>NSALDFLKHHLGAATPENPEIELLRLELAEMKEKYEAIVEENKKLK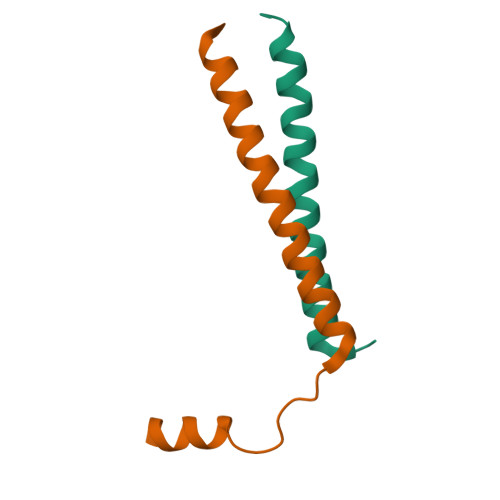AKLAQYE[4x]[[(2~{R},3~{S},4~{R},5~{R})-5-(6-aminopurin-9-yl)-3,4-bis(oxidanyl)oxolan-2-yl]methoxy-oxidanyl-phosphoryl] 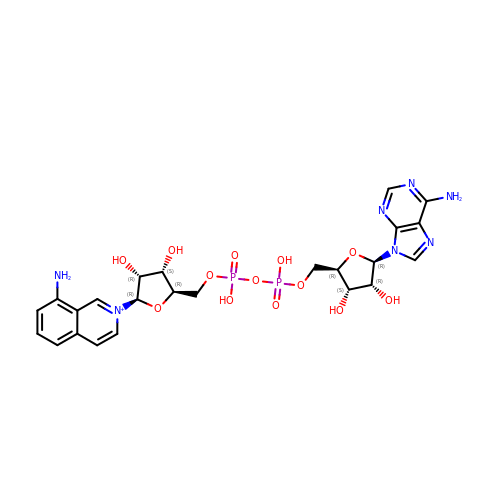[(2~{R},3~{S},4~{R},5~{R})-5-(8-azanylisoquinolin-2-yl)-3,4-bis(oxidanyl)oxolan-2-yl]methyl hydrogen phosphate | C24 H30 N7 O13 P2 | ZWKGBLKVIKZVCF-PAXFUWABSA-O>[2x]MVRIYTLTLA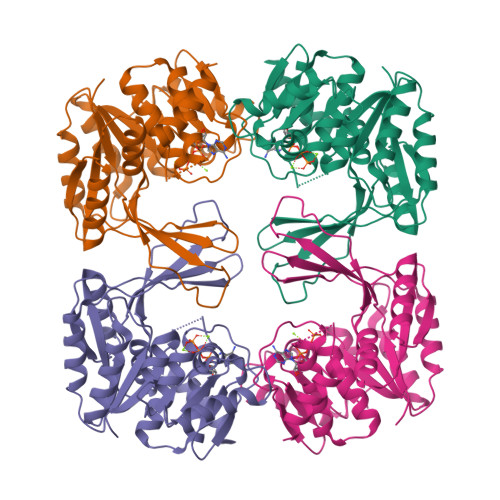PSLDSATITPQIDPEGKLRCTAPVFEPGGGGINVARAIAHLGGSATAIFPAGGATGEHLVSLLADENVPVATVEAKDWTRQNLHVHVEASGEQYRFVMPGAALNEDEFRQLEEQVLEIESGAILVISGSLPPGVKLEKLTQLISAAQKQGIRCIVDSSGEALSAALAIGNIELVKPNQKELSALVNRELTQPDDVRKAAQEIVNSGKAKRVVVSLGPQGALGVDSENCIQVVPPPVKSQSTVGAGDSMVGAMTLKLAENASLEEMVRFGVAAGSAATLNQGTRLCSHDDTQKIYAYLSR> SNSDVYAQEKQDFVQHFSQIVRVLTEDEMGHPEIGDAIARLKEVLEYNA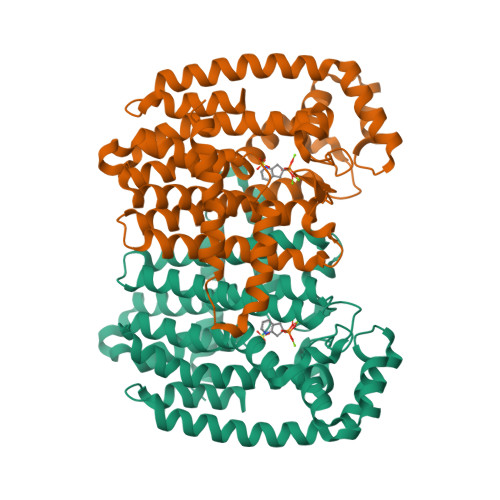IGGKYNRGLTVVVAFRELVEPRKQDADSLQRAWTVGWCVELLQAFFLVADDIMDSSLTRRGQICWYQKPGVGLDAINDANLLEACIYRLLKLYCREQPYYLNLIELFLQSSYQTEIGQTLDLLTAPQGNVDLVRFTEKRYKSIVKYKTAFYSFYLPIAAAMYMAGIDGEKEHANAKKILLEMGEFFQIQDDYLDLFGDPSVTGKIGTDIQDNKCSWLVVQCLQRATPEQYQILKENYGQKEAEKVARVKALYEELDLPAVFLQYEEDSYSHIMALIEQYAAPLPPAVFLGLARKIYKRRK Sirtuins are protein deacetylases and hydrolyze one NAD+ for each Lys residue they deacetylate, which links their activity to cellular energy levels. The conserved Sirtuin catalytic core comprises a Rossmann fold domain and a Zn2+-binding domain. The substrate polypeptide occupies a cleft between these domains, with the acetyl-Lys in a tunnel leading to the active site. Here, we show that resveratrol can directly activate the deacetylase activity of Sirt5 and inhibit the enzyme’s desuccinylase function as well as Sirt3-dependent deacetylation.

To investigate why resveratrol-like compounds activate Sirt1 and Sirt5 but inhibit Sirt3 we also solved the crystal structure of Sirt3 in complex with FdL1-peptide and piceatannol. The asymmetric unit of the Sirt3/inhibitor complex contains one monomer. As in the Sirt5/activator structure, FdL1-peptide and piceatannol bind in close proximity and directly contact each other. Peptide and piceatannol form crystal contacts to a symmetry-related Sirt3 monomer, resulting in π stacking interactions of the coumarin fluorophores of two FdL1-peptides and an interaction of the modulator with both stacked aromates. Piceatannol binds perpendicular to the coumarin rings, similar to resveratrol in the Sirt5/activator complex. The hydrophobic binding unit is completed by Phe294 and its symmetry-related counterpart Phe294*. Additionally, Glu181/181* participate in positioning of piceatannol by forming hydrogen bonds to hydroxyl groups in both rings of piceatannol. An overlay of the two complexes shows that both acetylated FdL1 lysines are bound in the hydrophobic active site tunnel, but the neighboring fluorophore/modulator pairs are differently arranged. As a consequence, the entire FdL1-peptide is shifted in the Sirt5/activator structure relative to the Sirt3/inhibitor complex, positioning the acetamide group deeper in the hydrophobic binding tunnel. Although the inhibitor contact to a symmetry-related substrate molecule in Sirt3 is likely a crystallization artifact, the Sirt3 structure shows again that the resveratrol-like compound can bind on top of the substrate and directly interact with the C-terminal peptide fluorophore, apparently influencing the substrate binding mode and presumably thereby inhibiting the subsequent reaction step.

> GSSDKGKLSLQDVAELIRARACQRVVVMVGAGISTPSGIPDFRSPGSGLYSNLQQYDLPYPEAIFELPFFFHNPKPFFTLAKELYPGNYKPNVTHYFLRLLHDKGLLLRLYTQNIDGLERVSGIPASKLVEAHGTFASATCTVCQRPFPGEDIRADVMADRVPRCPVCTGVVKPDIVFFGEPLPQRFLLHVVDFPMADLLLILGTSLEVEPFASLTEAVRSSVPRLLINRDLVGPLAWHPRSRDVAQLGDVVHGVESLVELLGWTEEMRDLVQRETGKLDGPDK>[4x]MPVRRGHVAPQNTFLDTIIRKFEGQSRKFIIANARVENCAVIYCNDGFCELCGYSRAEVMQRPCTCDFLHGPRTQRRAAAQIAQALLGAEERKVEIAFYRKDGSCFLCLVDVVPVKNEDGAVIMFILNFEVVMEKDMVGSPAHDTNHRGPPTSWLAPGRAKTFRLKLPALLALTARESSVRSGGAGGAGA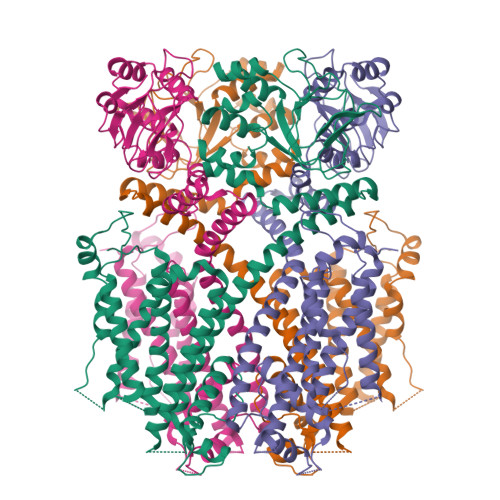PGAVVVDVDLTPAAPSSESLALDEVTAMDNHVAGLGPAEERRALVGPGSPPRSAPGQLPSPRAHSLNPDASGSSCSLARTRSRESCASVRRASSADDIEAMRAGVLPPPPRHASTGAMHPLRSGLLNSTSDSDLVRYRTISKIPQITLNFVDLKGDPFLASPTSDREIIAPKIKERTHNVTEKVTQVLSLGADVLPEYKLQAPRIHRWTILHYSPFKAVWDWLILLLVIYTAVFTPYSAAFLLKETEEGPPATECGYACQPLAVVDLIVDIMFIVDILINFRTTYVNANEEVVSHPGRIAVHYFKGWFLIDMVAAIPFDLLIFGSGSEELIGLLKTARLLRLVRVARKLDRYSEYGAAVLFLLMCTFALIAHWLACIWYAIGNMEQPHMDSRIGWLHNLGDQIGKPYNSSGLGGPSIKDKYVTALYFTFSSLTSVGFGNVSPNTNSEKIFSICVMLIGSLMYASIFGNVSAIIQRLYSGTARYHTQMLRVREFIRFHQIPNPLRQRLEEYFQHAWSYTNGIDMNAVLKGFPECLQADICLHLNRSLLQHCKPFRGATKGCLRALAMKFKTTHAPPGDTLVHAGDLLTALYFISRGSIEILRGDVVVAILGKNDIFGEPLNLYARPGKSNGDVRALTYCDLHKIHRDDLLEVLDMYPEFSDHFWSSLEITFNLRDTNMIPGSPGSTELEGGFSRQRKRKLSFRRRTDKDTEQPGEVSALGPGRAGAGPSSRGRPGGPWGESPSSGPSSPESSEDEGPGRSSSPLRLVPFSSPRPPGEPPGGEPLMEDCEKSSDTCNPLSGAFSGVSNIFSFWGDSRGRQYQELPRCPAPTPSLLNIPLSSPGRRPRGDVESRLDALQRQLNRLETRLSADMATVLQLLQRQMTLVPPAYSAVTTPGPGPTSTSPLLPVSPLPTLTLDSLSQVSQFMACEELPPGAPELPQEGPTRRLSLPGQLGALTSQPLHRHGSDPGS>MASMTGGQQMGRDPSQVVQVNDSMYGFIGTDVVLHCSFANPLPSVKITQVTWQKSTNGSKQNVAIYNPSMGVSVLAPYRERVEFLRPSFTDGTIRLSRLELEDEGVYICEFATFPTGNRESQLNLTVMAKPTNWIEGTQAVLRAKKGQDDKVLVATCTSANGKPPSVVSWETRLKGEAEYQEIRNPNGTVTVISRYRLVPSREAHQQSLACIVNYHMDRFKESLTLNVQYEPEVTIEGFDGNW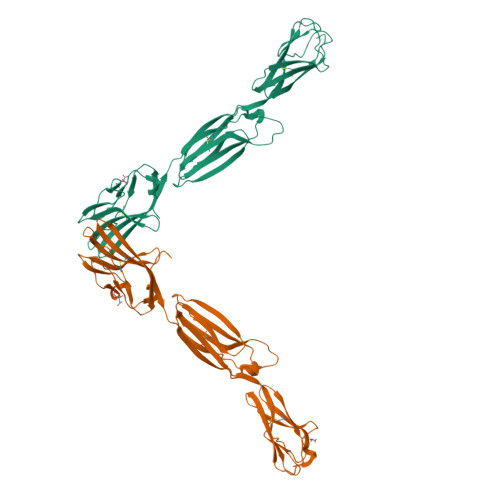YLQRMDVKLTCKADANPPATEYHWTTLNGSLPKGVEAQNRTLFFKGPINYSLAGTYICEATNPIGTRSGQVEVNITEAAALEHHHHHH[2x]> EGICALGGTSELSSEGTQHSYSEEEKYAFVNWINKALENDPDCRHVIPMNPNTDDLFKAVGDGIVLCKMINLSVPDTIDERAINKKKLTPFIIQENLNLALNSASAIGCHVVNIGAEDLRAGKPHLVLGLLWQIIKIGLFADIELSRNEALAALLRDGETLEELMKLSPEELLLRWANFHLENSGWQKINNFSADIKDSKAYFHLLNQIAPKGQKEGEPRIDINMSGFNETDDLKRAESMLQQADK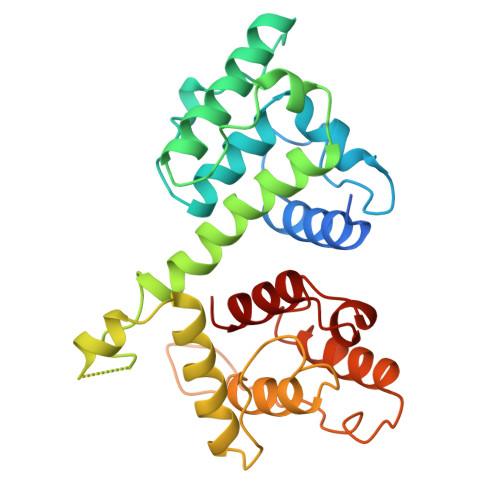LGCRQFVTPADVVSGNPKLNLAFVANLFN>[2x]MKTDFIMVPTAMPDEKMINYQLAIDGGEPVIPKANRKTIFPNIAKEDLFQMMISVQKPEEMVVSEFAEKYRQRVGAPYAIPTASGTSSLHLALVGAGVKAGDEVIVPAFTFIATAQAIVAAKAIPVFADIDPQTYCLDPRQLDKKVTARTKAVMPVHVHGLPADIDALASFCRQH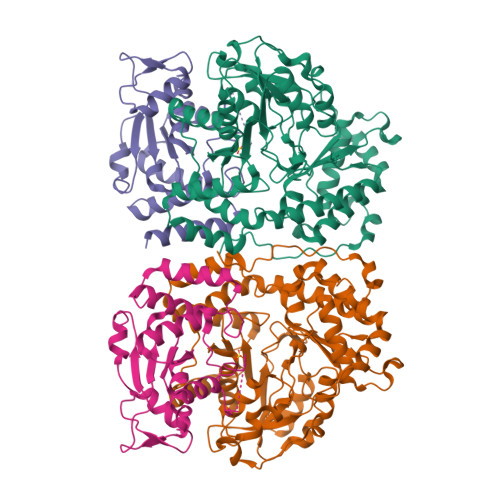QLALIEDASHAHSATLHGRYCGTFGDAAGQSLMADKNFPLGGEAGIAFFKERESYDRALAFLEESGLDYRMSWVAAAFGISQLDRLDYYDEIRQRNAQRLIDELATTRLFTGPMIPAAAKHSFNMFRIKINTALPEFKDIPEYKLKLALQQILNEEGVFAREWQNTLLPFHLPFQNKKGFGKGYPFFLGDSQEYKHEHFPNALQMLRSTLVLCRELRSPVEYEKLHSYIITFKKVDKNIQRVAEIASQIDDVPPYEKDARLGHHHHHH;>MGISKTSSDLSEQLFQVSFVLARVLTSGIIMSIEKNENELKGLENILKKTSSKQYAVTFNSISGAVIGSLWGQDIVYGEATNQQSLDEQQEKLFKWLGIGHSSLLPEPYTLHAINWGNISNLQKITHEEAHVTLLDFTKLGFGPCAVLLTNNETIYKKSERLKIFGAFDLRTMWTQRETEKEIKPGLQFNFRLSPLVGACIKMALIKMGLNKHHHHHH[2x]> MSCTTRRFIDEKEKLEYSRGYNQQELEASKLRKDFVKKYIVDFDTTLYKTQVERDWAYIAKREYRYEVQLKSIGYGGALANAVLLWRIYANKKMVFWPIPIVG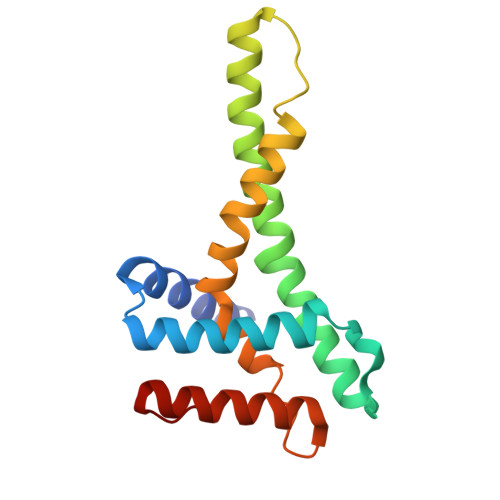ALGYLYFQPVFFQKSNKRFFDMCNVGEEYYLGRERNKILRECNKILNVEDF>MAHHHHHHMSAAAVQEIQSIEVTPLSAHIGAEIHGVDLTQKLEARQIAEIRAALLKWRVVFFREQFLTHEQHVAFSAQFGELTLGHPVFGHVEGHPEVYSISKYRKATRFEGQTLQRPWTGWHTDVTAAVNPPWASILRGVTIPPYGGDTQWTNLVAAYQKLSAPLRSFVDGLRGIHRFTPPAGASGTQAFVEAVEQRILVTEHPLVRVHPETGERALYVSPSFLKSIVGVSPRESQVLLELLWEHVTRPEFTVRFKWQAGSVAF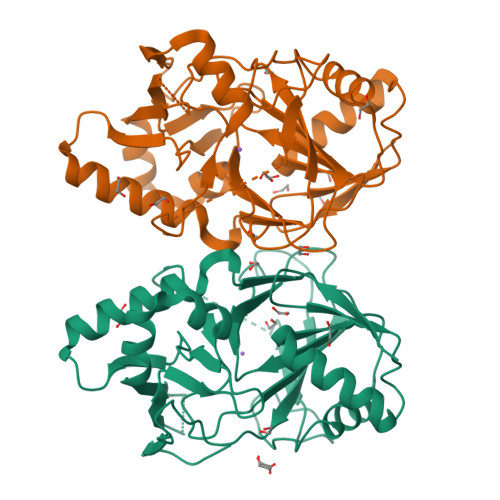WDNRATAHLAPTDIFDLDFDRQLYRTTLVGDVPVGPDGTQSVAIEGSPVSAAAAVALN[2x]The classical class I and class II molecules of the major histocompatibility complex (MHC) play crucial roles in resistance to infection and response to vaccines, binding peptides for presentation to thymus-derived (T) lymphocytes of the adaptive immune system as well as natural killer (NK) cells of the innate immune system. In contrast to humans and other typical mammals, the level of resistance to many infectious pathogens in chickens can be strongly determined by the MHC (that is, the BF-BL region of the B locus), at least in part because the chicken MHC is much simpler, with single dominantly expressed class I and class II loci. Virtually, all of the variation responsible for allelic polymorphism and thus for different peptide-binding specificities in different chicken class II molecules is located in the β1 domain of the β chain, encoded by either the BLB1 or BLB2 gene. We expressed BL2*02 linked to several Marek’s disease virus (MDV) peptides and determined one X-ray crystal structure, showing how a single small amino acid in the binding site causes a crinkle in the peptide, leading to a core binding peptide of 10 amino acids, compared to the 9 amino acids in all other reported class II molecules.

Soluble BL2 molecules from the B2 haplotype were expressed in insect cells using Baculovirus, with the peptide attached via a linker to the BLB2 chain [it should be noted that, in contrast to previous reports, the N-terminal positions of the BLA and BLB chains are likely identical to those of HLA-DR]. Of the 4 soluble BL2*02 molecules linked to MDV peptides that were expressed, the one with a peptide from gE formed crystals that diffracted to sufficiently high resolution to determine a structure. Overall, the structure of BL2*02 is extremely similar to BL2*19 and to the iconic mammalian class II molecule HLA-DR1, with root mean square deviations for Cα atoms of 0.684 and 0.878 Å, respectively. However, both chicken molecules have a four amino acid extension to the first loop and second β-strand of the BLA α chain compared to HLA-DR1. In stark contrast to all reported mammalian class II structures and to BL2*19, the BL2*02 has a decamer core, with the structure showing side chains at peptide positions P1, P4, P5, P8, and P10 of the core binding into pockets, so that the peptides that were first analyzed with a nonamer motif were reanalyzed for this peptide motif; the decamer sequence predicted by Gibbs clustering corresponds to the core sequence found in the structure. Compared to mammals and to BL2*19, the peptide in BL2*02 shifts the residues pointing up from the core towards the T cell from the typical P2, P3, P4, or P5 and P8 to P2, P3, P6, and P9, shifting register at P4. The conformation of the peptide bound to BL2*02 shows a polyproline II helix as in mammals but deviates downwards just at P4 and then returns to the helical conformation.

> ARHVLLQAEFYQRSEGPDKAWAQFGFHFDADELFHVELDAAQTVWRLPEFGRFASFEAQGALQNMAVGKQNLEVMISNSNRSQQDFVTPELALFPAEAVSLEEPNVLICYADKFWPPVATMEWRRNGAVVSEGVYDSVYYGRPDLLFRKFSYLPFVPQRGDVYSCAVRHWGAEGPVQRMWEPE;> ADRPQIESLSLNGVPNIFLSTKAGGGGSGGGGSGGGGSSAFFFCGAIFECHYLNGTERVRYLQRYIYNRQQLVHFDSDVGKFVADTPLGEPQAEYWNSNAELLENIMNIADGSCRHNYGILESFTVQRSVEPKVRVSALQSGSLPETDRLACYVTGFYPPEIEVKWFLNGREETERVVSTDVMQNGDWTYQVLVVLETVPRRGDSYVCRVEHASLRQPISQAWE>[4x]MPAPEAPTSTLPPERPLTNLQQQIQQLVSRQPNLTAGLYFFNLDSGASLNVGGDQVFPAASTIKFPILVAFFKAVDEGRVTLQERLTMRPDLIAPEAGTLQYQKPNSQYAALEVAELMITISDNTATNMIIDRLGGAAELNQQFQEWGLENTVINNPEPDMKGTNTTSPRDLATLMLKIGQGEILSPRSRDRLLD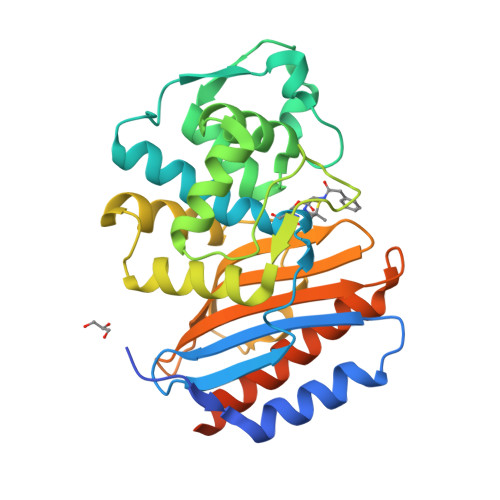IMRRTVTNTLLPAGLGKGATIAHKTGDIGIVVGDAGMVDMPNGQRYVAAMMVKRPYNDPRGSELIRQVSRMVYQAFEKLSPPEQKLISEEDLNSAVDHHHHHH We assessed the performance of these methods in the identification of sulfur hydrogen bonds within the active site of the enzyme Alkyl hydroperoxide reductase E (AhpE) from Mycobacterium tuberculosis. To test our approach on structural coordinated atoms in space, we used the active site environment of the peroxidatic sulfur of peroxiredoxin AhpE, a single cysteine enzyme. AhpE reduces H2O2 to water but no H2O2 is present in the active site of the AhpE structures. Method 3, however, only finds the interaction with the water molecule, not the Arg116. It is predicted that stabilization of the Cys45 thiolate by Arg116 will promote its nucleophilic character, so that this Cys represents a catalytically active state of the enzyme.

The crystal structure of AhpE shows 2 dimers per asymmetric unit, which are denoted chains A and B17. Accordingly, we decided to use both chains in our analysis, because the cysteine environment in each is distinctly different. In chain A, the side chain of the conserved arginine residue (Arg116) is oriented away from the cysteine and directed outwards to the flexible β9-α5 loop, whilst in chain B it is turned inwards to the active site cysteine. To improve protein stability during MD simulations, we realized that a re-refinement of the models of the AhpE structure was needed (see supplementary). After this re-refinement operation, we repeated the simulation with the newly refined structure for chain A and found that after 30 ns the helix α2 remained intact. Importantly, a gauche minus conformation was found for the peroxydatic Cys45 in the active site of chain A after re-refinement, which is in line with the conformation reported for most of peroxiredoxins. In chain A with Cys45 modeled as a thiolate, the sulfur has four direct H-bonds, while in chain B five H-bonds were found. In the active site of chain B, most H-bonding interactions are intra-protein, involving the side chains of Thr45, Arg116, and the backbone amide of Cys45. In the case of chain A, however, the H-bonding network is much more dependent on water molecules, which, in their mobility, provide a less stable H-bonding environment. Beyond that, our results confirm that chain B, where the conserved Arg116 is located in the surroundings of Cys45 active site, is the reactive conformation for H2O2 reduction.

>HMLNVGATAPDFTLRDQNQQLVTLRGYRGAKNVLLVFFPLAFTGICQGELDQLRDHLPEFENDDSAALAISVGPPPTHKIWATQSGFTFPLLSDFWPHGAVSQAYGVFNEQAGIANRGTFVVDRSGIIRFAEMKQPGEVRDQRLWTDALAALTA[4x]>VVTYNTLIDGLCKAGKLDEALKLFEEMVEKGI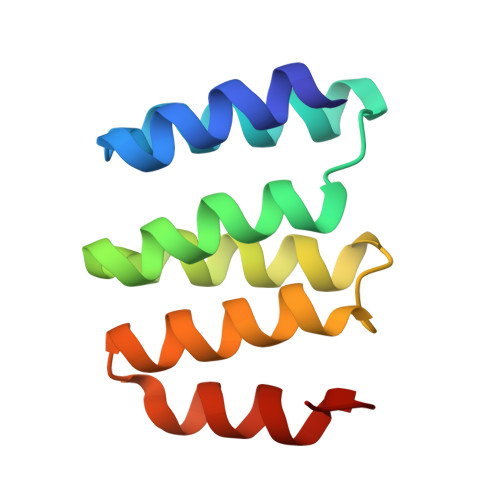KPDEFTFSSVLKACARLGALELGKQIHGYVIKSGFESNVVVYNALIDMYSKCGLLEEARKVFDEMPEKD[2x]>SRKTYTLTDYLKNTYRLKLYSLRWISDHEYLYKQENNILVFNAEYGNSSVFLENSTFDEFGHSINDYSISPDGQFILLEYNYVKQWRHSYTASYDIYDLNKRQLITEERIPNNTQWVTWSPVGHKLAYVWNNDIYVKIEPNLPSYRITWTGKEDIIYNGITDWVYEEEVFSAYSALWWSPNGTFLAYAQFNDTEVPLIEYSFYSDESLQYPKTVRVPYPKAGAVNPTVKFFVVNTDSLSSVTNATSIQITAPASMLIGDHYLCDVTWATQERISLQWLRRIQNYSVMDICDYDESSGRWNCLVARQHIEMSTTGWVGRFRPSEPHFTLDGNSFYKIISNEEGYRHICYFQIDKKDCTFITKGTWEVIGIEALTSDYLYYISNEYKGMPGGRNLYKIQLSDYTKVTCLSCELNPERCQYYSVSFSKEAKYYQLRCSGPGLPLYTLHSSVNDKGLRVLEDNSALDKMLQNVQMPSKKLDFIILNETKFWYQMILPPHFDKSKKYPLLLDVYAGPCSQKADTVFRLNWATYLASTENIIVASFDGRGSGYQGDKIMHAINRRLGTF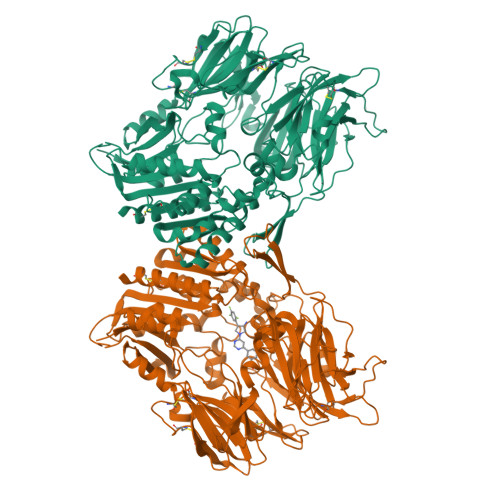EVEDQIEAARQFSKMGFVDNKRIAIWGWSYGGYVTSMVLGSGSGVFKCGIAVAPVSRWEYYDSVYTERYMGLPTPEDNLDHYRNSTVMSRAENFKQVEYLLIHGTADDNVHFQQSAQISKALVDVGVDFQAMWYTDEDHGIASSTAHQHIYTHMSHFIKQCFS[4x]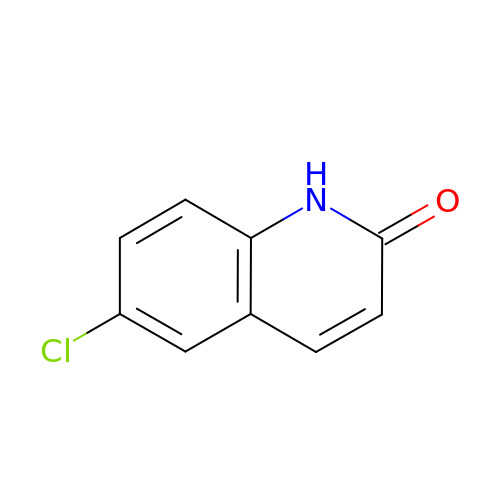6-chloroquinolin-2(1H)-one | C9 H6 Cl N O | OJEBWFGRUPIVSD-UHFFFAOYSA-N>[2x]ETQQRCVTATDYDTFVSERFGSIIQAVQTFTDSTKPGYAFIAAKPKSGLYLTTVQREDIKNYLKDYNLAPITPSIISPNYLFIKTNLKVTYALNKLQESEQWLEGQIIDKIDRYYTEDVEIFNSSFAKSKMLTYVDDADHSVIGSSATIQMVREVQNFYKTPEAGIKYNNQIKDRSMESN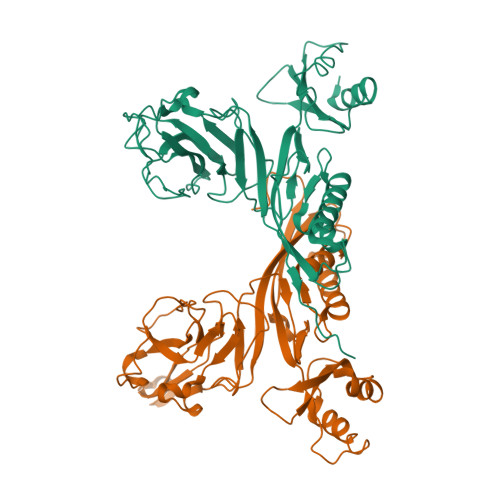TFSFNSGRKVVNPDTGLEEDVLYDVRIVSTDRDSKGIGKVIIGPFASGDVTENENIQPYTGNDFNKLANSDGRDKYYVIGEINYPADVIYWNIAKINLTSEKFEVQTIELYSDPTDDVIFTRDGSLIVFENDLRPQYLTIDLEPISQLEHHHHHH>[2x]SNAQPKDVPVTFTAITQGVWMHTSMKHMENWGHVPSN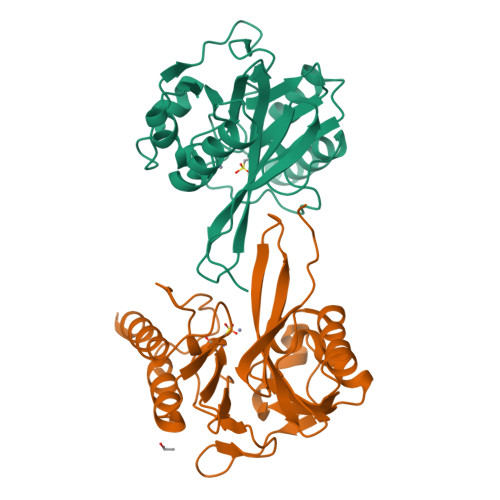GLIVEKGDFSILVDTAWDDPQTAQIIEWSKDTLKKPIRWAVFTHAHDDKMGGVAALRQQGIVTYAAADSNRMAPQNGLTPAEHDLIFDSEHSTSVLHPLVIFDPGPGHTRDNIVVGLPEQGIVFGGCLIRPSGSTSLGNTADADLAHWKTAVLAVAQRFAEAQQIIPSHGPMAGRELFELTAQLAEKASIPST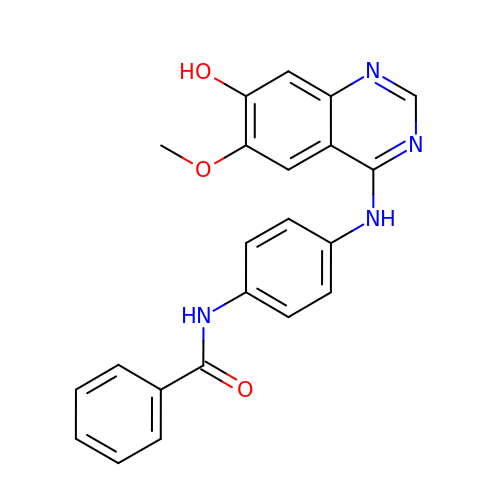N-{4-[(7-hydroxy-6-methoxyquinazolin-4-yl)amino]phenyl}benzamide | C22 H18 N4 O3 | FRAOYGZBTRQIIP-UHFFFAOYSA-N Doublecortin-like kinase 1 (DCLK1) is a multi-domain bi-functional protein that belongs to the protein kinase superfamily and the doublecortin (DCX) family within the microtubule-associated protein (MAP) superfamily. Doublecortin-like kinase 1 (DCLK1) is an understudied bi-functional kinase with a proven role in tumour growth and development. Multiple isoforms of DCLK1 exist, generated by alternative splicing. Here, we report the crystal structures of DCLK1 kinase domain in complex with DCLK1-IN-1 and its precursors.

To understand the structural basis by which XMD8-85 increased inhibition of DCLK1 and to elucidate its retained pan-activity against ERK5 and LRRK2, we solved the structure of DCLK1-KD (residues 372-649) in complex with XMD8-85 to 2.5 Å. In DCLK1-KD:XMD8-85, the sulfate coordination is no longer maintained. Despite this, the activation loop is visible in an open conformation with the first three conserved activation loop residues Asp-Phe-Gly (DFG) adopting a classical DFG-in conformation. In this conformation, the DFG phenylalanine packs into an hydrophobic grove and contribute to the intact regulatory and catalytic spines, indicative of an active conformation. This active conformation is further confirmed by the presence of the canonical salt-bridge interaction between the conserved αC helix glutamate (Glu436) and the invariant β3 strand lysine (Lys419). The interaction of XMD8-85 with DCLK1-KD results in two hydrogen bonds interactions within the ATP binding site. The secondary amine (N2) in the linker between rings D and C of XMD8-85 acts as a hydrogen bond donor for the backbone carbonyl oxygen of Val468, and the  pyrimidine nitrogen atom (N5) in ring C of XMD8-85 acts as an acceptor for the backbone amide -NH of Val468. Notably, the amide carbonyl oxygen of the diazepine ring B participates in a network of water-mediated hydrogen bond interaction with the invariant Lys419 and αC Glu436 that play a critical role in nucleotide binding. The N-methyl amide substituent at position R4 on the diazepine ring B confers affinity for DCLK1. This R4 N-methyl group  appears to form favourable vdw interactions with the gatekeeper residue Met465 (on β5) located deep in the ATP binding site, as well as Ala417, Val449, and Glu466. Firstly, the ortho methoxy substituent in ring D in XMD8-85 is likely better accommodated in DCLK1 than the bulkier ortho ethoxy substituent of XMD8-92 as this bulkier substituent would be expected to cause unfavourable contacts with E406 of DCLK1; secondly, protonation of the N-methylpiperazine of XMD8-85 at physiological pH would enable an additional favourable electrostatic interaction with Asp475 of DCLK1, which is not possible for the 4-hydroxypiperidine substituent of XMD8-9228.

>[2x]GSGEEVSEEGFQIPATITERYKVGRTIGDGNFAVVKECVERSTAREYALKIIKKSKCRGKEHMIQNEVSILRRVKHPNIVLLIEEMDVPTELYLVMELVKGGDLFDAITSTNKYTERDASGMLYNLASAIKYLHSLNIVHRDIKPENLLVYEHQDGSKSLKLGDFGLATIVDGPLYTVCGTPTYVAPEIIAETGYGLKVDIWAAGVITYILLCGFPPFRGSGDDQEVLFDQILMGQVDFPSPYWDNVSDSAKELITMMLLVDVDQRFSAVQVLEHPWVND>TTNTDSFTFSKFKPNQPNLKKQGDATVTSSGTLQLTKVDKNGVPDPKSLGRALYASPINIWDSKTGVVASFATSFRFTIYAPNIATIADGLAFFLAPVSSPPKAGAGFLGLFDSAVFNSSYQTVAVEFDTYENTVFLDPPDTHIGIDVNSIKSIKTVKWDLANGEAAKVLITYDSSAKLLVAALVYPSSKTSFILSDVVDLKSVLPEWVSIGFSAATGASSGYIETHDVFSWSFASKLSFXXXXXXLDLASFLVAN[4x];>[4x]TTNTDSFTFSKFKPNQPNLKKQGDATVTSSGTLQLTKVDKNGVPDPKSLGRALYASPINIWDSKTGVVASFATSFRFTIYAPNIATIADGLAFFLAPVSSPPKAGAGFLGLFDSAVFNSSYQTVAVEFDTYENTVFLDPPDTHIGIDVNSIKSIKTVKWDLANGEAAKVLITYDSSAKLLVAALVYPSSKTSFILSDVVDLKSVLPEWVSIGFSAATGASSGYIETHDV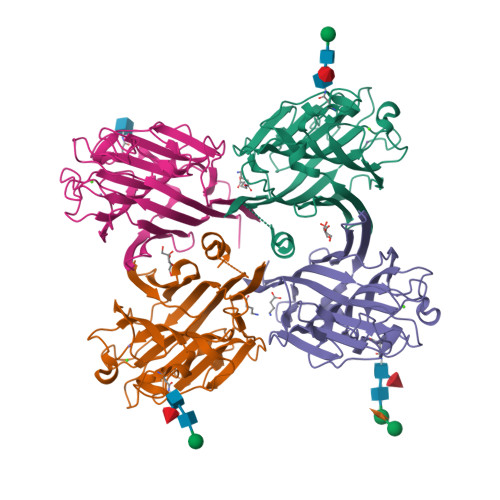FSWSFASKLSFAA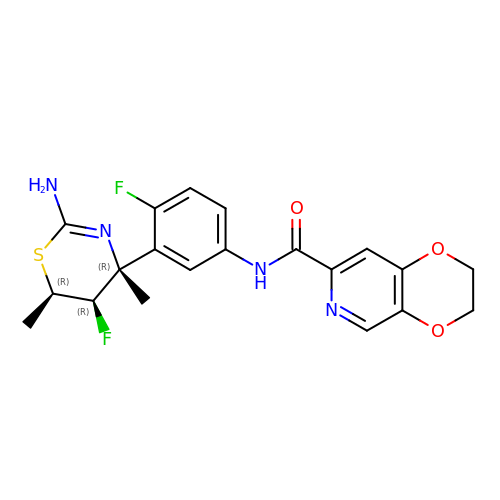N-[3-[(4R,5R,6R)-2-azanyl-5-fluoranyl-4,6-dimethyl-5,6-dihydro-1,3-thiazin-4-yl]-4-fluoranyl-phenyl]-2,3-dihydro-[1,4]dioxino[2,3-c]pyridine-7-carboxamide | C20 H20 F2 N4 O3 S | LQVIUEMPEFSVOL-CPRIZNHFSA-N>MRIKLIIVEGKTDESFFKVLLEKLYGFREAKKLTPEFPIGKWGFRIGEHPLVLEKDNIALVIIHAEGKQRIPKVLKSVLDSVKLGLLNVEEVYVVRDVDEGNDVFEWVLSFLREREVRVDNGAIVTEGVKIYPYGMGNLTLNEPFVKEKKELELSLAYLAKLDGILEKYRGSMRALSQDKGDKLTPKDVMHILSIANDYTGDCLSGLYEKYIGIMIHRNRELL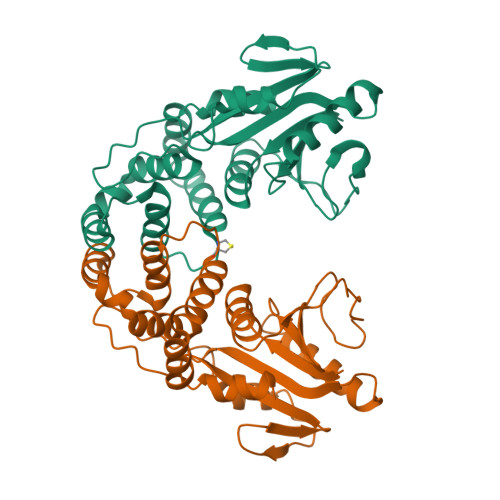IRFLSEVNLLPLLERMVG[2x]>[4x]MKSNGCRYGTHRVIEPKGVLPQPAKILNNDMSEIWDNEMLIDVIRLNIDSASFHQIKNKLIAQGHQDLEKAFAEHAIELTNRTGKHKNEDTGSGGMFIGRVAAIGDKFEMKEEVKVGDKIASLVSLSLTPLKINKVKKVLLDKDQMEIEGQAILFSSGVYAKLPDDLDENLALSVLDVAGAPAQVERLVKPDDTVVIIGANGKSGIL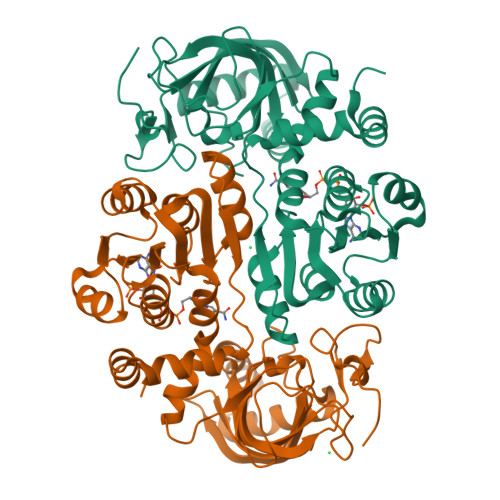CNAVAKERAGICGKVIGVVRNENYIPTCKATGCDEVILAQATDAITIQKEVSRLTNGKMADVVINVVNTEDTELPSIMAAKDRGMVYFFSMATSFTKAALGAEGIGADVDMMIGNGYAHHHSEIALDLLRRNSVLMKIFKERYAEHHHHHH> GAQVSRQNNGTH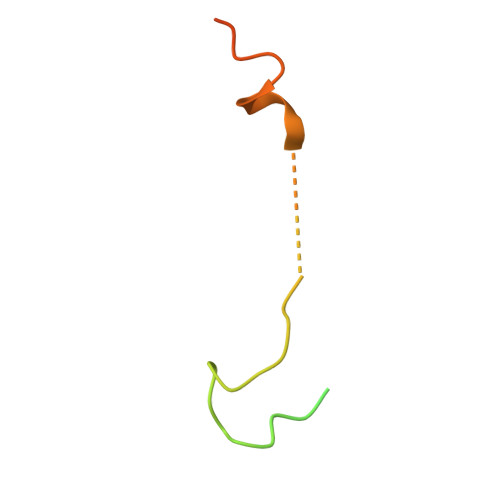ENGVTASNGSVIKYFNINYYKDSASSGLSRQDFSQDPSKFTQPLVDTLTNPALM> AGCGCCGUGGCGCAGUGGAAGCGCGCAGGGCUCAUAACCCUGAUGUCCU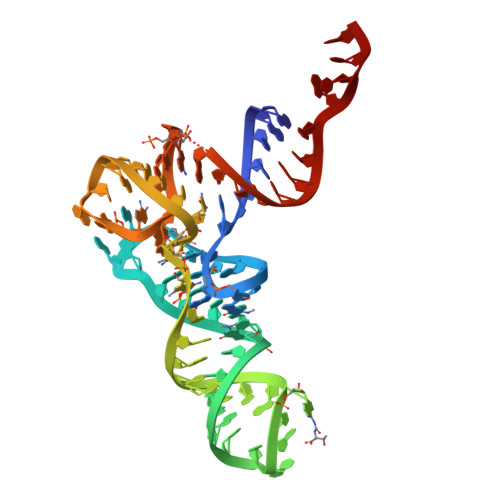CGGAUCGAAACCGAGCGGCGCUACCA> MGKYFGTDGVRGVANSELTPELAFKVGRFGGYVLTKDKQRPKVLIGRDTRISGHMLEGALVAGLLSIGAEVMRLGVISTPGVSYLTKAMDAEAGVMISASHNPVQDNGIKFFGGDGFKLSDEQEAEIERLMDEPEDKLPRPVGADLGLVNDYFEGGQKYLQFLKQTADEDFTGIHVALDCANGATSSLATHLFADLDADVSTMGTSPNGLNINDGVGSTHPEALSAFVKEKNADLGLAFDGDGDRLIAVDEKGNIVDGDQIMYICSKHLKSEGRLKDDTVVSTVMSNLGFYKALEKEGIKSVQTAVGDRYVVEAMKKDGYNVGGEQSGHLIFLDYNTTGDGLLSAIMLMNTLKAT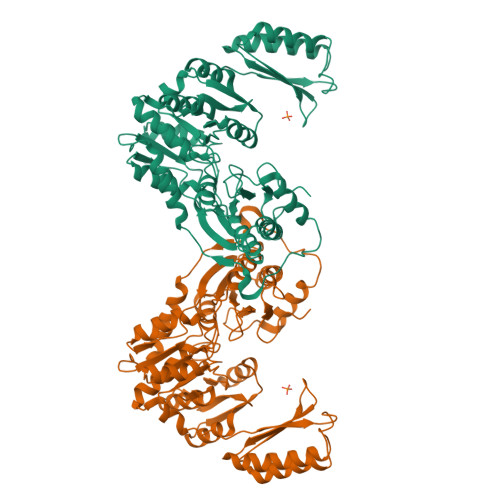GKPLSELAAEMQKFPQLLVNVRVTDKYKVEENEKVKAVISEVEKEMNGDGRILVRPSGTEPLVRVMAEAKTKELCDEYVNRIVEVVRSEMGLELVPRGSSGLEHHHHHH>[4x]AGEMIEAPSQVLNFEEIDYKEIEVEEVVGRGAFGVVCKAKWRAKDVAIKQIESESERKAFIVELRQLSRVNHPNIVKLYGACLNPVCLVMEYAEGGSLYNVLHGAEPLPYYTAAHAMSWCLQCSQGVAYLHSMQPKALIH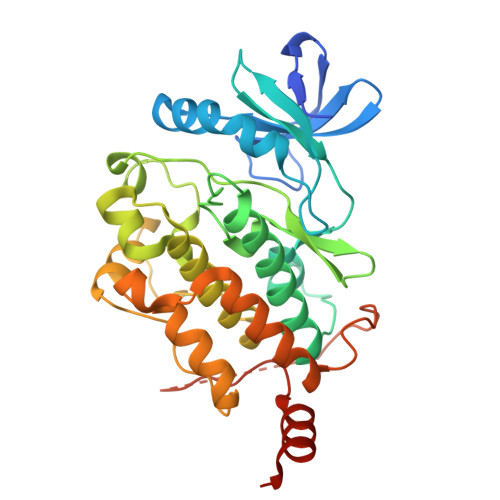RDLKPPNLLLVAGGTVLKICDFGTACDIQTHMTNNKGSAAWMAPEVFEGSNYSEKCDVFSWGIILWEVITRRKPFDEIGGPAFRIMWAVHNGTRPPLIKNLPKPIESLMTRCWSKDPSQRPSMEEIVKIMTHLMRYFPGADEPLQYPCQHSLPPGEDGRVEPYVDFAEFYRLWSVDHGEQSVVTAP>MVLYFIGLGLYDERDITVKGLEIAKKCDYVFAEFYTSLMAGTTLGRIQKLIGKEIRVLSREDVEANFENIVLPLAKENDVAFLTPGDPLVATT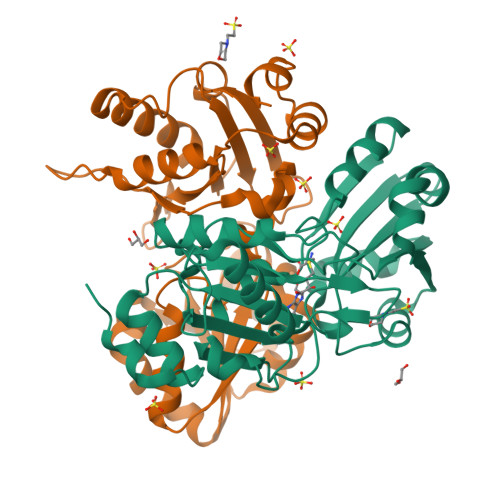HAELRIRAKRAGVESYVIHAPSIYSAVGITGLHIYKFGKSATVAYPEGNWFPTSYYDVIKENAERGLHTLLFLDIKAEKRMYMTANEAMELLLKVEDMKKGGVFTDDTLVVVLARAGSLNPTIRAGYVKDLIREDFGDPPHILIVPGKLHIVEAEYLVEIAGAPREILRVNV[2x]> ADGKYAQKLFNDLFEDYSNALRPVEDTDKVLNVTLQITLSQIKDMDERNQILTAYLWIRQIWHDAYLTWDRDQYDGLDSIRIPSDLVWRPDIVLYNKADDESSEPVNTNVVLRYDGLITWDAPAITKSSCVVDVTYFPFDNQQCNLTFGSWTYNGNQVDIFNALDSGDLSDFIEDVEWEVHGMPAVKNVISYGCCSEPYPDVTFTLLLKRRSHHHHHH;> GCCSDPRCRYRCR

Nicotinic acetylcholine receptors are the prototypic members of the Cys-loop family of pentameric ligand-gated ion channels, including also the 5-HT3, GABAA, and glycine receptors. The α9 subunit of nicotinic acetylcholine receptors (nAChRs) exists mainly in heteropentameric assemblies with α10. RgIA, on which the present study is focused, is a 4/3 subclass α-Ctx (containing four and three residues in loops 1 and 2, respectively), and is highly selective for the α9α10 nAChR. This neuronal nAChR subtype has two stoichiometries, the (α9)2(α10)3 and (α9)3(α10)2, and is mainly expressed in the hair cells of the cochlea and in a variety of immune cells.

The crystal structure of the complex of the deglycosylated human nAChR α9-ECD in complex with the C-terminally amidated α-Ctx RgIA was solved at 2.26-Å resolution. Upon binding, RgIA is buried in the (+) side of α9-ECD and shares a common orientation with other previously determined α-Ctxs bound to AChBPs. Its central helical domain protrudes toward the binding site, while its N- and C-termini are located at the bottom and top of the binding site, respectively. The most profound interactions of RgIA with the (+) side of α9-ECD involve its aspartic residue at position 5 and its arginine residues at positions 7 and 11. RgIA-Asp5 forms a H-bond with loop-C α9-Tyr192, RgIA-Arg7 forms H-bonds with the carbonyl oxygen of loop-C Pro200 and the hydroxyl group of loop-A Tyr95, while RgIA-Arg11 makes a salt bridge with loop-C Glu197. Additionally, RgIA-Pro6 makes van der Waals interactions with the loop-B Trp151. In addition, in the crystal structure of RgIA, an intramolecular salt bridge between Asp5 and Arg7 was observed, also missing from its NMR structure. Instead, the salt bridge between Asp5 and Arg7 of RgIA is most probably induced by its binding to α9-ECD, since this is also apparent in the crystal complex of ImI with AChBP, while lacking from its varying NMR structures. Moreover, since the complex of the monomeric α9-ECD with RgIA superimposed very well with the complexes of the pentameric AChBPs with ImI and other α-Ctxs, this study showed that the (+) side of the α9-ECD alone is adequate to determine the orientation of the bound RgIA. The Ki values for the two α9-ECDs, differing in their glycosylation state, were slightly different, with the deglycosylated α9-ECD (the one co-crystallized with RgIA) having 2.7 ± 0.3 μM, and the glycosylated one having 13.3 ± 1.5 μM.> ANVVQRNSPSWGLSRISSKKSGATDYVYDSTAGEGIVIYGVDTGIDIGHADFGGRAEWGTNTADNDDTDGNGHGTHTASTAAGSKFGVAKKASVVAVKVLGADGSGTNSQVIAGMDWAVKDSKSRGATGKSVMNMSLGGAYSRAMNDAAANVVRSGVFLSVAAGNEAQDASNSSPASAPNVCTIAASTNSDGSASFTNFGSVVDLYAPGK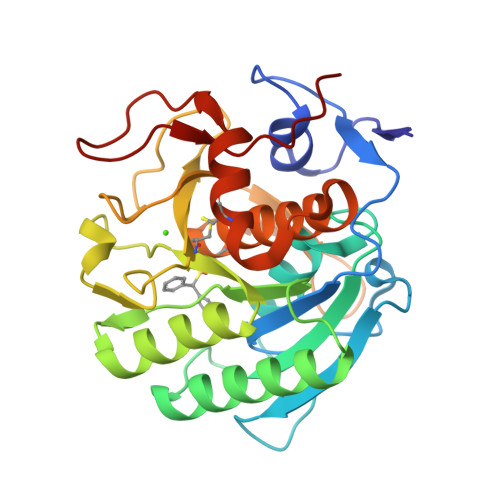DITAAYPGGGSKTLSGTSMAAPHVAGAAAYLMALEGTTTSSACARIVQDAITKISGAPKGTTTKLLYNGING> VC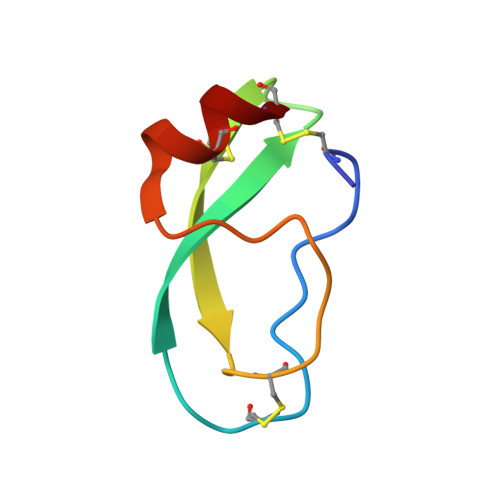SEQAETGPCRAMISRWYFDVTEGKCAPFFYGGCGGNRNNFDTEEYCMAVC> KENICIVFGGKSAEHEVSILTAQNVLNAIDKDKYHVDIIYITNDGDWRKQNNITAEIKSTDELHLENGEALEISQLLKESSSGQPYDAVFPLLHGPNGEDGTIQGLFEVLDVPYVGNGVLSAASSMDKLVMKQLFEHRGLPQLPYISFLRSEYEKYEHNILKLVNDKLNYPVFVKPANLGSSVGISKCNNEAELKEGIKEAFQFDRKLVIEQGVNAREIEVAVLGNDYPEATWPGEVVKDVAFYDYKSKYKDGKVQLQIPADLDEDVQLTLRNMALEAFKATDCSGLVRADFFVTEDNQIYINETNAMPGFTAFSMYPKLWENMGLSYPELITKLIELAKERHQDKQKNKYKID

Ddl is essential for staphylococcal growth and produces d-Ala-d-Ala dipeptide which is incorporated into peptidoglycan to cross-link the peptide side chains of neighboring glycan strands. Ddl has two d-Ala binding sites and one ATP-binding site, and DSF experiments were conducted with various combinations of these ligands. We demonstrate that acetate anions bind to and inhibit d-alanyl-d-alanine ligase (Ddl) activity in S. aureus.

To gain further insight into the mechanism of acetate inhibition, the X-ray crystal structure of a Ddl/acetate complex was obtained using co-crystals of Ddl and acetate. The crystal diffracted to 1.9 Å and data were consistent with a P 2 21 21 space group possessing one molecule of Ddl in the asymmetric unit. One acetate is positioned within the adenine binding subsite of the ATP binding site and the other acetate ion is positioned in the second d-Ala binding site. The acetate ion in the ATP binding site interacts with the side chain of Lys177 and the backbone nitrogen of Val216. Also, the methyl group of acetate forms van der Waals interactions with the side chain of Leu145. The acetate ion that binds to the d-Ala binding site forms a bidentate polar interaction with the side chain of Arg291 and a hydrogen-bonded interaction with the backbone nitrogen of Gly312. These two residues are conserved in Ddl homologs and previous structural data clearly illustrate the crucial role these residues play in d-Ala binding. The acetate-bound structure shows conformational differences compared to the previously published ligand-free and ADP-bound structures. Interestingly, this loop is well ordered in the acetate-bound structure described here, which gives the first view of the S. aureus Ddl ω loop and the interactions it may form with substrates or inhibitors. The ω loop is shifted towards the ATP binding site and repositions the conserved Tyr246 side chain within the ATP binding site, which likely hinders the binding of ATP.>GLSAEQIAVLQEQGFELRDEGWEFGMSSKVLFGNNLDRLNPDSRNTLTKIARA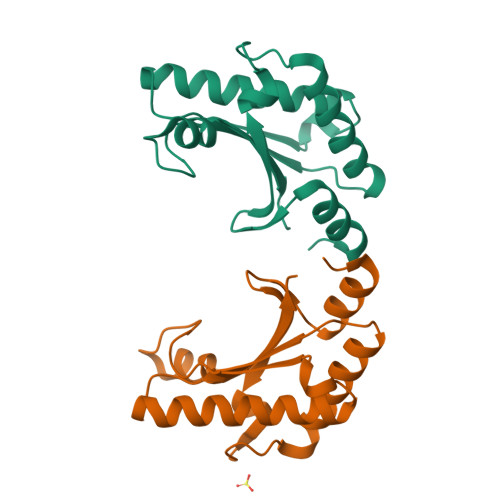LLAVDIDKVRLEGHTDNYGDEGYNQKLSERRAESVAAVFREAGMPAANIEVRGLGMSKPVADNKTRAGRSENRRVAIIVPAE[2x]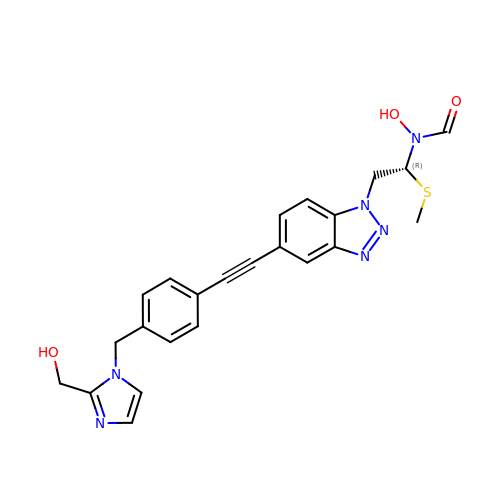N-hydroxy-N-[(1R)-2-{5-[(4-{[2-(hydroxymethyl)-1H-imidazol-1-yl]methyl}phenyl)ethynyl]-1H-benzotriazol-1-yl}-1-(methylsulfanyl)ethyl]formamide | C23 H22 N6 O3 S | PDKPBTURFVUWEE-HSZRJFAPSA-N> MSNLFRSLASSMRALSLAAPRATAVNTTKTVVSTHQTRCLSQGLLSRHICTPMCSHNRPVAVCQSAKNGLQSKQQSRGMKVHSAIKKRCEHCKVVRRKANKRQNGYLYIICPANPRHKQRQGYR;> MSTCQQVARPLVRCLRQTGPGAATCSTRSVAVAAVRPFSSTPMRKEEGATTTTTTSPVDSTTTPPPLPSATEAKATVADTVVGGPELGSRRRRAALATTGNLPFEQLPYQCFQDARKILQQDRAAKIAQIVKETEKIKLIEARDASEFEGGEAAKQTRIKSLRKYIEELKILADINDPEVKRRFEDGRGDMTKPVYRFMAERRWRSMDYKIIAQRISQFHVVPDLLPAFDPTMDVKLSFRGYQVSPGAILDSRVTEVAPTLRMQVFDKGERLLTVVVIDSDVPDVTHDNFKRRCHFLAANIPWDPSKTVLSLRSVGDRVEGDVGKPWLPPFAQKGSPYHRLNVFVLEQKPGAKIDGEALKKHLENRENFSLKGFREKFDLEPVGFNLFRSEWDEGTAEVMERHGIPGAEVEFKRQKFASLKPPRKARGWEAKRQKPKYKSLWKYVKRIA;> MVSATKKPVSAMSAKNSTRHRKVSHKVTKTIATAKSQVISNKAMKIRTKSWKDMPSPKRRRRINAMVDELRLQGNVKMPKPGKSTYKAGGGERVRLVKAASTLPTPPLTPPVLSKPTGSASQSKGDLKPKRPTPEKKRSVSKRDVERFFLSTQTSTRRRENTPIHAPIMSSTFTSLRGLATRLFAGGARPSPSSLLLPNKPATAALPTAIQHQQTASYASKGKSGPPAGMFSGQKAGSKKSKGPKQVDPRIINILRHFAVLSPKRIPPPLRFGRNRYLRHWTIHRAWLLFRRQQREQRERILMQQHQSMSNACEELRNTEGPGTRETGYLYRVAMLKNGVYGLKSIPIEYASRALVETPGRQAWNHEWKR;> MQPTRILQGLKYRKLRLTTKDVNKGFYKGNRTGSMGTHTSYGTYKIDYTKVRTYVCPDLTGFKLTPFVSKTIRPVHDQFPGDKLGPKNPATYLARWKSENGLD;> MTVKALTQISSAGRNGVGAFVLQCKKLDIHYSDWAGSSRGMNGFIKSLLPKFAAANPQIEFVVSPRPAKHPILMGHYINGRTKAICVRNMEPLEILKKAELLRDASGEKPQKFKKPVTSTNPSVRGVWSPYHGQGMAV;> MKRIATPSLTSRLLVAARSGVSPATAAIRSRSAISVRSQSTAALAQHDASHDLNNDRFPPLEPLPPAAESLPSPLPERALTSAKLAALHARLNLSPKIPLQTLARTLVDASADENPQFNNANLAFVGQTLINYHIAEWLLCKYPRLPQGILFSAMKAYAGPKPLLQIARSWGVDTAAVPGGEVDPGLLQFDALKPGVAITNFGYKRTELAYLEKFKWRRGMASRVVLDDDFGDVVRSDPKVAADLEKAMEEQDQDKTPDEEEAEMVANEQDQDVSYDRYGNPDTRAAAERAHAYFVRAVVGAIYAHCGREAAKAFVKAHIMSRTLDIAKLFEFKYPTRELAALCAREDFEPPVARLLSETGRQSRTPVFVVGIYSGSDKLGEGAASSLDHARFKAAMNALKAWYLYSPGENPRVPSDMLEEGAKPWTPAYIDMGEVISR;> MSASSRGAALLRSQQRSICLQCRNQTRVLAPAGVTSAPRRFYSAEASATATATATATTTTTLPPPHPPVTTSTGTHAATSTSSQIYRIKSGVILTRPPLLTRDLTPFEESFYFYQKRLNERLTAPFRKDFYFKKDTAADLDWRIKLKERHGVPAKDIGRYNPRGRMAWNDEVLVGSQTSSRKHMVEKLLADAEMRVSEDGEEIPAEDRVPVEKPMPRRTEADEKGDVKRLDRALDKTLYLVVKKKADKEGEEAKWMFPTGVVPTDEGLHETAARILAESAGVNMNTWIVGRVPVAHHVVRPVFGQKDGALLKKGEKIFFLKGRIMAGQADLTDNLHDLVDFKWLTQEELRSTLAEEYFHSVKGMFAER;> MFRSTFFGLSRAIVQPATPLTVRAAFQSRFYSAAAAASQPTTTATTTTPLQQQQQQQPTTQPTTPIQTQTGAAPTESTKPVAKPYLVGRAWTQRLPVYHLAKRGGNKKLTQIKKVQGDGQALRRDLAQFLGLEVKEVRVKVPTGHLEVDGHRREEIVKFLDGLGF;> MRRIPRIPSTASALCSSSSSVASTSAAPLRTLRAAADSSSICQSCSFSTQTSATRNRVWQNTVQTQRRCASTVTETTPEAPVAAAAAETATESTETVEQQRKRKGGFFETQRQVNLVLPGQPTRADAPEKIRDPNYEPATSGAGLQEIGGMSDWWSKPEHFRDGGKQFEYQGFAPQEKITDPRLLKVILRRALAEGLALKKFGANPKNPADMASIIGNGDHWQRTVSVEMCRGENGELSLKNESDLQKVWILMRNAAEKTYYQREWQEEINRLRSLGEKEQAKQLLEEGKKLGYRLKSEEGSLVKLTVDEAVELRKSWNNDWKEAIIRDPVVKFYAAKRIQKMTGHILSDGKLTSIQTVANFMDALVTPPKPKKLAEQIEQSSILPELPNVKVYPRRVTPVDKERMVGRWKVIQKELQKRELPVLGTGNHGKYVELKWLGSKQ;> MAALTPSRSVFASTCKTIAQQCSRRPVAVQQLAAVPVARQVSSSSAVQQEQDASGTSSSQQPRPRWSYTPERMKGPGFSLNLVKDPRRKQWMVNSDPAKLDAFYDAFLGQGGSRMLSEETKWLAVTHKSFDYGRRGYNTRLAFLGRQIIALETTRSILTSPVLNEPIVDKYGRTPYNHAALANIDKLIYTQPLDIMDKTKIARMGIDFGLLTVMRWKPRMPEDLESSGVVVVLNSTLFAIIGAISLEKGAAVAQRIVREKILKRLGA;> MLQPQFRPLLAGTASFAQTVLGRTVARCYATKAATQSASSTSTSNTSKDAKAKIVTPYVRDAGMMRTYKPHTPGIRHLKRPINDHLWKGRPYLPLTFPKKGQSKGGRNHSGRVTVRHRGGGHKRRIRMVDFERWIPGPHTVLRIEYDPGRSAHIALVKEEATGRKSYIVAADGMRAGDVVQSYRSGLPQDLLDSMGGVVDPGILAARTCWRGNCLPVSMIPVGTQIYCVGSRPDGKAVFCRSAGTYATIISKEEETREDGTKVMTGKFVNVRLQSGEIRRVSKDACATVGIASNIMHHYRQLGKAGRSRWLNIRPTVRGLAMNANDHPHGGGRGKSKGNRHPVSPWGTPAKGGYKTRRKSNVNKWVVTPRVRNMGVRRNKKTT;> MAPRLPARCWRQLSLVERSATHTTTTAAASSLLLAGRTTPTFSASSPSTVFPSLLPQITKRGVKYGWSTLPKRSRPTRFNQVTQGLPAPTSGPAAALKRREKTTPLRTGVLAVKKGMTVFMGRTGARIPCTVLQLDRVQVVANKTRAKNGYWAVQVGLGERRAENVGAPQLGYYEAKGIPPKQTLAEFKVRNQDGLLPVGVQLFPDWFHVGQVVDVRGITRGMGFAGGMKRHGFAGQEASHGNSLNHRTIGSVGGSQGSGSRVLPGKKMPGRMGAQQHTVQNLPILMVDNELGIVVVKGAVAGHKGAVVKVQDAVKKAPPPEEFVEATKQLLNERFPDAEEKLQAARKLHLELKEARRQGLIDSLIKNGLTEKADGNAAVEASA;> MAGKGLKSLNEAMNALSIASKSCRALPMRQSSILPCRRSMASVATPPAANITRSVSEPWQPITNVPVTVYSFPELEPRSLESYSARHLHLPLRRDILHLAVIYEGDSTRRGMASTKTRYEVHGSHKKMSPQKGTGNARRGTRQSPLMKGGGKTFGPKPRDFSTKLNKKVYDLAWRTALSYRYKRGELIVTEDGLDLPLPNDFLWLAGGGKLSRELEDGYVRKWVHEFMTSLNWGKEAGRTTFITGDKRPNLFTGFELAGAEGRALELWDVDVKDLLETGRIVIERSALKEMIEDHQSDLVTRVAVQGLRQKGPNLGEVLVRAPRY;> MASLRGVSRSARALQPFSAQFAVRRCASTQTGAGAAAATPKSNIPDLAELETRSALDAPIPSEEDKKEFRPWKRAADRKARLPSSRYQYHPPKYNRGPLHPIQSPPSSDPIARDFVPGPFNMPRLKETFRTVMASDLMTLAYIHTPPGTPKKEPTERLRAWEGDSPYFANRARRAPRGAPELPIRERDISFRNIPEIKEITVSTFVPLGLKNPDLLIVARAVLLAMTGTMPEMTRSKNNVVQWQLQANKPAGCKTTIYGNAAWEFMDRLIHLVLPRIKDWKGVPASTGDGSGNVQFGLNPEDVQLFPEVECNYDMYPAKMIPGCHIAIKTTATSDRQAKLLLQSLGVPFYSN;> MFAPSRRRVLEAVASSSSSPVVTLPGFLVPAFQQTAGAAARRNFSATTTRPSKLGRTPLSIPPGVEITIGEPFVKRDMTQWKQQPKRKITVQGPLGQLEMDIPDFIKIDHDAEARRATLSVANRDEKEQREMWGTTWAYLNRFIMGVSEGHTAVLRLVGIGYRATIDTRPEKEEYPGQQFVCLKLGFSHPVEMGVPKGMKASTPQPTRILLEGINREQVMTFAADIRRWRVPEPYKGKGIFVNGETIKLKQKKIK;> MSQTVGATRLAYSRVWHHISAVTPHPTLSTIKAPSEAITPPSLGRLASRIATILMGKHKPIWDPSTDCGDYVVVTNCAGLYTTGHKKWRKTYYRHNTRPGSLQAITMDALMEKHGGAEVLRKAVSGMLPKNRLRDKRLARLKAFEGDAHPYKENLVRFGGKVVGAPGWEEAVKAIREADMERL;> MIQLKTMLNCIDNSGAALVECAMVVGQKRHASIGDRIVVVVQKQRGADSAGMAASSAATKVKRGDIRHAVVVRTKQKVQRRDGSVVRFDDNACVLINKAGDPIGSRINGVVGQELRKKKWSKILSMAPMQA;> MPPRLPLAQAARCCQASLTARPSVPASSPTSSLISLFAALSVQTRSASILASLSDNRGAYHKRIRKGRGPSSGYGKTAGRGTKGQKAHGHVKPWFQGGQTPLIVSHGRKGFVNQFAADMSELNLEKLQEWIEAGRIDPTKPITPKEIIKSGIIGSSIKDGIKLLGRGKESFKIPVTITVSRASASAIEAIEAAGGKIVTRFYTKESLKRLVEGKSLHTDKPLPVGKEHVEEILAQARSLKKKYYRLPDPTSRWDIEYYRDPAHRGYLSHQLAPGESPSLYFKVPTGGEKVKVVRADKVKASKTGDVASEKLF;> MKHNASSALLSAFQGLRISSSATPFRAASLATSAVRRPIAPTPVSVASHVRLFSATAIQAGSWLEPNLNRKKKMMKGRPRVPTGGSTKGTTVVWGDYGLRMRDHHRRISAQQLKLAEDTIKQRLRGQKYRLYKRVACNVGVYVSGNEMRMGKGKGSFDHWATRVAVNQIIFEIRGQLHEQVIRDAFRLAGHKLPGLYEFVKKGDPPVVGITKLEDGLTVEDLKNPRKKLLMPEITQSAASTSSTAAPPS;> MAGAHVKYRHLSRSSAHRQALLRNLVTSLIKNETIHTTYPKAKEAQRLAEKLITLSKRDTETARRSAQGILYTPDQLLPKLFGEIRERYANRPGGYTRVLRTEPKDQYSQAPSAILELVDGPKDMRFAMTAATVARDREQKTESTDLTKKNMDKVTRFRKDGMRAFEDMVASLRDMKFTAGAINPKEWKKLDR;> MNVTASLSRRPLGCLKAGLCQSLIRGYATAVAASTTQSTGALPDHNFFRIADKHTKKTRTAFAVFTPPKSPTTLPPSSVVTKSKAFKIANSKLPPLMTKPPSDPMPLLTQQQIARMDPTGARTALFSKARHAARVGDVLMVTHRRGGEPFAGVCLAIRRSGIDTAILLRNHLGKVGVEMWYKIYNKNVAGIEIIKRRAKRARRAKLMYMRQPKHDMGSVEQYVFAWKKMRKVLSSKGLTGGVGGGGGKQKGQESKKKN;> MSRALLRSVLELRTPVTRLPPSFLLPFRPAARFLHQTAQQVEPTSQSDAAAAAATLLKASPPKVTTATTPEAPAAVPTSTPFSQQPPISQQVKELLPVLAAQPGHYTTIHIHGKPYLVTEGDTVKLPFKMPGVAPGDVLRLNRASVIGSRDLTLQGAPYVDERLFECRAIVMGTESEPMRVMIKKKRRCRKKKHVFSKHKYTVLRINQLKINDVSSL;> MSLNVPSRRLLKSAPSSANALVPALQSLSINTRSIHTTPSQQWSLFGWGKQKVEERNKVKEELKQSELARTRKPTQEEIFERVRGRLEGDSIFADTTPSSQLAAEQDKHKDWATASAEKKLAAAHAKDQTPTGISLKKDHLVRVVDPDPRSRVRWERKMVIRKLQRGTDPWSVEPKAERIARTERKLVYKTGYLPTSVKKLVHLSRQIRGKTVSEALVQMQFSKKKMAKEVKTELLRAEAKAIVTRGMGLGKAAAAAAQKETGAEPVKIQTKDGKHLEIRDPTRIYVAETFVNKGFTRGVELDYRARGRVFKMNKPTTTMTVVLKEEKTRIREHQERVAKKLRQGPWVHLPDRPVTSQRQFYSW;> MASVAKTGAEALRNAPFRVGKKQIFLPNHVITFVRPLPKQPPNLATFIVPLEFNKLDLRDYLYHVYNVEVTGVRSFVNQRMHEQRHGDVGNWRRPKSQKMMIAELAKPFVWPKPPAEDAREAFDYAMWKKQKTAQEQDTKFQGIRAQGEVVPPSQFEVTKDRKAIKARQSKFLSGEETWAPGKVNAFLNSKIVPEEEGWSEVEENLPLDESAESAAEESSSKGSETRQ;> MDKLLRRVRMAEGMVARRAQRKNALLKRITERKQNKKNGEAFTEAIQQRKAAVEARNEDWMLGPLAPRRELDEITLSNGNFFGSLSPTRALLESEVSEEERKARVAWCGSPKFLCIAPGDRVVVIEGHHKDLIGTIEKLNTRNMTVEIQSEKLKTNTTVPQFMQNDADKPVTQIYARLPISSVRLVHPLKDPQTGEYRDVIIRELRPRNIVHDRPTRTRSMRRFVPGENIIIPWPKQEPIKREDQPADTLRIDVDEKTFVPTLFRPPAPQQVLDELRNKYSIFRTRHTPEYIAKKEQEEQEKEAKKSAAKAMLTPVQEYNRKQRELRRARGQPALTEEMLAKIGEVVARNKLGHHQAPKVKEETVAQIEKAVEQLSLGGGQEDAATTTSPEQPKVV;> MHLAQLRQPLTRAAANSCHSVCRLPTTHSSVSATAILSEQFAHLRIGPSSSNVAVEGRRYASVKAQGAYRLKPKRTIPKKLGAKKTGDQYVIPGNIIYKQRGTLWHPGENTIMGRDHTIHAAVAGYVKYYRDPQLHPDRQYIGVVFNRNDKLPYPKDAPRKRKLGLVAVPRKVEEVEKPTMSASGLPLFVTRHETIEIPPPAVTTPAAAGKAVKGQGARVSASGAAAVPASSSTISASASSNSNNGGSSVIAELIKEKLAARAEYNARQSALRKLQQQKMLARRGTRVLRLMNNYSYRETNWEIGRLIGDPGSVPGTEKVGSRKAKFRARRRRRNTFLLGIKERKLAKADRREEYRRRVREKREQRLVQRKEFLAKQREAKKAREGGAAAEKSEKKEVKAEKPAAAAPKVEKPKAPEAAKKESKPKVEEKKAAAAEPKKDSKTEKKD;> MSSFLVRPFCLRATTTTTTTTTTTALVQQQLRALTTTTALTYHQPRVPSSAIPIPNVSGRVPLPDSTPVPEDFKIEIPSYPYGPRRVYHQSNTGLYGSALIRFGNNVSKRNEIKTRRKWRPNVQQKRLWSKSLGVFVRTRVTTRVLRTIDKVGGLDEYLLGHKAARVKELGPWGWMLRWRIMQTPEIRERFAKEREALGLPPRREEDEEKSLEEQLREFQVAGIQFAEGKAPKTKGQLKEEADRLIKKSETEEFGLGQEEDLFMKEEPKPTKMA;> MASPAALRPSMGAIMQTCRSAATAPKVAVAVPVRALSTSAALLKRHKYPTARVTRDNSKQRGESALRKSGTRWKLSVSDEPLPEPVPREELPPIQVDENHGLWDFFYDRETVAMAPLEHTKHGRAWTVSELRKKSWDDLHRLWWVCVKERNRIATANWERTKSELGFGLAEANERDRNVKQTMRGIKHVLTERFYAWEDAVKLAEQDPEIDLSNPENPYTPSTFLEAEETAEGAEASETQSTTTEIDPTTIPSSKSQAEAPRV;> MSFFRITLHRSAIGLPKRTHGVLAALGLRRRNQTVFHPVEPQFAGMLMKVKELVRVEEVPHRLTKRELKDERKPDAGFVVEKQVRRFIPGVGVQDEVDFSKVVEELKAQKVENVEGVEKMVVEGGAVVRDGKRAGDLGVRTRSDWEVIGKMKSVLPKVKAL;> MSSKLPTTLLRRPSALPSTTTYTAYSASRPTPPSCTAHGAQGQQIRNATFVPRHRRPYQFTQLVQLSDGSTFTVRTTMPTALYKSAKDSRNHLLWQPSDKSLKNVELDEAGKLAAFRERYGRGWDLDAKMTPEEEAAAAAALAAGGGAGVPGGKAAKKAAEEALLAKKKKEEEEAAKKAAEAEEADPFDSLTDLISGYATENMNPGLNFKETRHYGKKK;> MAAMTAAAAAPAMRLFNPSTFFQTLRTQRFGVPALNFAVPAAAISLLPSIPSLLEDIWEGILRAVPKKKTSHMKKRHRQMAGKALKDVTHLNRCPACGNLKRMHHLCSTCLGKLKGFMDRNGGSNAKAY;> MAKKAKSRIINVRLISMAMTGYFYTFTRPRTSLPMSMLKYDPIVRRKVLFLEQKRKGRS;> MSRIFSSALQAVFKPSAFLPKTATRSFSILPSLRPATLSSTPSTIFRAPNAITAPSASPSATTGIDGEVLDLLSASSLISSHPALSGLGSQIRCGPRPTMSGATRLVQKRRHGFLSRVKTKNGQKTLKRRLAKGRLRLSA;> MEASLSLFRPVATCCRRVALSSSSSSSQKAAAVAGISVRYQSTANRTKRMLNIPPHESFLNVPVEGDRIIFNPPSSEASVYHTPFKFLPRSDPRRRANIYKLFKPPQAPITTPESSSTDAAAADQHGDLPPVLYNPTKSYNVTPEQVEEIRELRAKDPKKYSVTYLSNKYNCTKVFIMMCTQAPREHQEQHKLARARTAENWGPRRAAAKLDARRRKEMLHRGEI;> AATVKQHVQLALSLPPRLRTFLARYPPASILPAGADPETHKTPYQEESPNPFMPTKHPITGKWHNPKYSLRRQAELVKLAQEHGVEELLPFTRKLNEEKLRKRVELGLRVKGTGVGEKVKGHKHERTLVAKMEKRREAMLAMPDLIREWKKVGKRNWTKFPK;> MFGAFRFTNPLSGGLLWKIPWRMSKFQKLRQRRRLRAVDNVVATIENALAKKGETVKAVERWRAEMPTEAEMLPKDKYTIFDRKEKRYRKGIHKLPKWTRVSQRVNPPGY;> MNSVTTSTIGRLAFGVSRLSAVTNVAGAVRHASTHPTTAIPKPTTAVLKTSPLAEETAVELKSPSRLQLKSEPGNKGNPKGHGDRIWAFHHIEQGQVIYSTKPVISHQHLIRQQPFTGKNLVPRKIRKDYWRPLAMIELAGKDQGAVGRSVYQKLREFKKRHELDWANEAEEGRKLMHKSKRERGQELNDQKPNSVADMAAVLAGAGKGNLMWQVSRLGSSSELVGEIKKASGAVEKGAVVDVKRQLRRATVYWTNEQDKFHAREWSDNVSHEVGIPGEAEKKRMPIRMSSE;> MSLRLSRPAVRGLGSAIKSSRISSRSAALLVPSTSTSAFSTASPQRAAAAGHLRLPDDYVPPTQPPSARPVDTRKSQLLRTYTSMLRSTPLMLIFQHNNLTAIEWAAIRRELSLALSNVPVPEGAPDITSKIHLQVVRTRIFDVALKTVEFFDPSTVEPTTATTATGTKVPATYNHDLSKHAWKAVKEATKNTEAVEKTVYGQLAPLLVGPVAILTLPSVSPAHLGAALSVLAPSPPAFPAPSRKKNPGYYDLTCQSGLQKLLLVGGRIEGKAFDYDGIKWVGGIENGIEGLRAQLVHMLQSAGMGLTSVLEGAGKSLWLTMESRRSVLEEEQNPKKEGEGEEEKKE;> MSKAAKGGAGGVEQVVKLIVGAGQASPSPPVGPALGSKGIKSMDFCKEFNARTAHINTGTPMPVRVTVRPDRSFHFDVRTPHTSWLLLNAAEAPIGKGGKRKGASNPGKEVVGTVSLKHVYEIAKIKQSELRLSGLPLEGLCRAVIYQARSIGINVIP;> MLTRFITDVSTRFNPFSAKAKAARLFLSFLPPNARSNGMNITTQLLPRNSTETPLLYVKFKDGKEMNLDVENMGIKSIVEEVDRHSRILQKQADLNDG;> MICRTCLRRASGFARPAAAAATRPMVAASSRAAFSTTFSVCTPPAATPAAAAPATSTAEAGLAPVPGAATTEQAKAAISSCPAGTKLNGLNYFKNKADPVALPDEEYPEWLWRCLEVQKKTDDAADADAGDEFSKSKKQRRLAMKRARAQEAKILASGDLEALAPKIPLQKQSVNLPGAVNGGVQDAVLADEKREELRKAMRKERKAKIKESNYLKAM;> MSATPAVLRASACSACRFSALRLFVSSFASPRAPLPVARTRVLSPTAPYSTFRPSPRLLASPSSEEHAEPAAQEQPNKTEDAQAEASTEANNEGGADVPWYLQVDAPTHPTLVHEPPPLPDIPEGSPKLMEPLVKFVSDELGMDDLKLLDLREIDPPPALGPEVLMLFGTARSERHLHVSADRLVRWLRNRGVTAKADGLLGRNELKTKLRRKARKAKLLGTTGLPSGADDGITTGWICVNLGTLGWSDMEMEFKDEKGVTSGFGVPQSGTTLVVQLMTETRREELALEKLWSGILRRSLERQDKIAGKLPEASFTTSPDTVSGQSFSPSPIRSSGRNRKRPDRLYFSTSARQHAAAVDVSQTDLATAMAGWEYSNASPSTIDNLLAQDTDSKVQLLIQMQEYLSSLPRDQALSAVSLCEDGSPSTFMRLFNRAIENLPSAQAWEARLWVEKAARALQHPDHDLARLGDLIQEMKLSGAANVSREKFVDLLRMIFAIPETTDAGVRQQASLSMDVIDMLFSRGEKVIEYDVVVAVIESLLQTRARPPEARRLLSQFEDLLSEAQMDCPTEDEIIRLLDVYANHRAWDKFWNVWRVFPRHCERRTERMYTKVYERIAAEDHQGMATDALRWCVEEMWHEQPPVRVTAAMLKALEACIRIADPEAESLAKDIDDRISDAQYMDREFVRLWLTLHGSAAWGA

Protein synthesis in mitochondria supports bioenergetics of eukaryotic cells and is executed by dedicated mitoribosomes. To provide a representative reference for studying protein synthesis in the mitochondria of fungi, and to reveal how the mitoribosome functions in coordination with its translation partners, we determined structures of the translating mitoribosome from the representative fungal model organism Neurospora crassa. The fungal mito-ribosome consists of 78 different proteins, 23S and 16S rRNAs. Forty-eight bacterial orthologs are extended, and 30 proteins are mitochondria-specific.

During 3D classification, we recognized a minor population of the particles corresponding to the isolated mtLSU, and subsequent processing resulted in 3.03 Å resolution reconstruction from 24,142 particles. Fitting the mtLSU model revealed an extra density that appears as a protein element forming a heterodimer with uL14m. We identified the extra density as Atp25, an ortholog of the bacterial ribosome silencing factor (Rsf), for which there is no high-resolution structural information in complex with a ribosome. We observe only the Rsf/MALSU1-related part of Atp25 on the mitoribosome, confirming the function in the assembly of the mtLSU. In addition, rRNA at the interface (38-ES2, H63, H67-71, H80, 82-ES6, H101, PTC) appears as unfolded. Further, the L1 stalk changes to a conformation that is more flexible and the density for bL9m next to L1 stalk is absent, whereas all the other mtLSU proteins are present. Atp25 presents only in the class with the missing bL9m and unfolded interfacial rRNA that affects the L1 stalk. Atp25 bound to uL14m sterically obstructs the binding of the mtSSU by preventing the formation of bridge B8 with its globular domain. The steric block spans ~25 Å and would clash with h14 of rRNA and the N-terminus of mS26 of the mtSSU. Therefore, the eviction of Atp25 must take place during the final stages of maturation to alleviate the steric hindrance on subunit joining.The first identified human member, ClC-1, is essential for maintaining the permeability of Cl− across the plasma membrane of skeletal muscle fibers, gCl, accounting for approximately 80% of the resting membrane conductance and assuring precise neuronal control of muscle contraction. Despite distinct roles as passively conducting Cl− channels and stoichiometrically coupled secondary active Cl−/H+ antiporters, members of the CLC family share a common homodimeric core architecture, with each subunit harboring an independent ion translocation pathway. In addition, the complex gating processes that regulate CLC channel activity remain elusive, with only a single available structure of a channel member, namely, that of bovine ClC-K. Each CLC monomer has a gate that operates independently from the other (also known as “protopore” or “fast gate”), structurally attributed to a specific glutamate, “GluGATE”. Here, we have determined structures of full-length human ClC-1 using single-particle cryo-electron microscopy (cryo-EM), exploiting a purified protein sample that displays Cl−-dependent single-channel–derived ion conductance.

For structural characterization, sample in the presence of 100 mM Cl− at pH 7.5 and in the absence of nucleotides or antibodies was initially employed. Assessment of the 3 major cryo-EM maps obtained in our structural classification reveals different arrangements of the CBS domains, suggesting intrinsic domain flexibility at pH 7.5. Therefore, the CBS arrangements seem to correlate with slow gating, being rigid at low pH in the presence of nucleotides and more flexible at higher pH in the absence of nucleotides, bringing to mind a mechanism that has been proposed based on electrophysiological data. The complete effects of such putative rearrangements are, however, not demonstrated experimentally by our structures, because they remain closed also at the higher pH (determined from particles in detergent environment).

>MEQSRSQQRGGEQSWWGSDPQYQYMPFEHCTSYGLPSENGGLQHRLRKDAGPRHNVHPTQIYGHHKEQFSDREQDIGMPKKTGSSSTVDSKDEDHYSKCQDCIHRLGQVVRRKLGEDGIFLVLLGLLMALVSWSMDYVSAKSLQAYKWSYAQMQPSLPLQFLVWVTFPLVLILFSALFCHLISPQAVGSGIPEMKTILRGVVLKEYLTMKAFVAKVVALTAGLGSGIPVGKEGPFVHIASICAAVLSKFMSVFCGVYEQPYYYSDILTVGCAVGVGCCFGTPLGGVLFSIEVTSTYFAVRNYWRGFFAATFSAFVFRVLAVWNKDAVTITALFRTNFRMDFPFDLKELPAFAAIGICCGLLGAVFVYLHRQVMLGVRKHKALSQFLAKHRLLYPGIVTFVIASFTFPPGMGQFMAGELMPREAISTLFDNNTWVKHAGDPESLGQSAVWIHPRVNVVIIIFLFFVMKFWMSIVATTMPIPCGGFMPVFVLGAAFGRLVGEIMAMLFPDGILFDDIIYKILPGGYAVIGAAALTGAVSHTVSTAVICFELTGQIAHILPMMVAVILANMVAQSLQPSLYDSIIQVKKLPYLPDLGWNQLSKYTIFVEDIMVRDVKFVSASYTYGELRTLLQTTTVKTLPLVDSKDSMILLGSVERSELQALLQRHLCPERRLRAAQEMARKLSELPYDGKARLAGEGLPGAPPGRPESFAFVDEDEDEDLSGKSELPPSLALHPSTTAPLSPEEPNGPLPGHKQQPEAPEPAGQRPSIFQSLLHCLLGRARPTKKKTTQDSTDLVDNMSPEEIEAWEQEQLSQPVCFDSCCIDQSPFQLVEQTTLHKTHTLFSLLGLHLAYVTSMGKLRGVLALEELQKAIEGHTKSGVQLRPPLASFRNTTSTRKSTGAPPSSAENWNLPEDRPGATGTGDVIAASPETPVPSPSPEPPLSLAPGKVEGELEELELVESPGLEEELADILQGPSLRSTDEEDEDELIL[2x]A HEPN (higher eukaryote and prokaryote nucleotide binding) nuclease Las1 and a polynucleotide kinase Grc3 assemble into a tetramerase responsible for rRNA maturation. Las1 and Grc3 are highly conserved proteins and have recently been identified as core enzymes involved in processing and removing ITS2 spacer, which is a key step in the synthesis of 60S ribosomal subunit. Recent studies have demonstrated that Las1 is an endoribonuclease that contains a HEPN (higher eukaryote and prokaryote nucleotide binding) domain responsible for rRNA processing. Grc3 is a polynucleotide kinase responsible not only for Las1 nuclease activation, but also for nonspecific phosphorylation of the 5′-OH of the 26S pre-rRNA produced by Las1 cleavage, providing a signal for further processing by Rat1-Rai1 exonuclease.

Cleavage assay indicates that ScGrc3 can activate ScLas1 nuclease well for ITS2 cleavage, while CjGrc3 exhibits relatively weak activation ability for CjLas1 nuclease. To better understand the differences in the mechanisms of Grc3 activation of Las1 between different species, we also solved the cryo-EM and crystal structures of full-length CjLas1-Grc3 complex at 3.39 Å and 3.39 Å resolution, respectively. To be noted, the crystal structures were solved by molecular replacement method with the cryo-EM maps of Las1-Grc3 complexes. Structural superposition shows that the conformations of all Grc3 domains and Las1 HEPN domains are almost identical in the two complexes, while the conformations of Las1 CC domains are significantly different. Notably, compared with CjGrc3-bound CjLas1, ScGrc3-bound ScLas1 has a more compact catalytic pocket, which may explain why ScLas1 shows better ITS2 cleavage activity than CjLas1 in the presence of Grc3. In addition, His130 in the ScLas1-Grc3 complex active site and the analogous His130 in the CjLas1-Grc3 complex active site adopt two different conformations, which are similar to the conformations of His142 of CtGrc3-bound CtLas1 in two different active states. This observation may also provide a structural rationale for the activation of ScLas1 and CtLas1 by Grc3, as well as for the fairly weak activation of CjLas1 by CjGrc3.

>MHKSAFQALQGDIPTYEVNSSDEQDSDQDEEDVEQPSEPMHRLVSAPAASIHIEESKYISSNFSFDDDNTIYGHDYVIFGLKSNQNLIVKGQFVLEIQRGAIDINGVIYHSGVEPMKFINPSSSSIPLIQATQVLNSSLLENKESQENQHLFTPGYKSVIKLTNLDTHLESIGRVCPLFKNLFWQFDNFFAEDSLRLLDQYELAFSDYTFYPITKPDNTVSVIKHKNWMDVIKSLTELYSNDQSIKVIVIGGKNSGKSTFLRLLVQHMLSPTLQQLPINFMDLDPGQPEYSGTDCISLSKISEVQHGNHLSLTSTDSTQCHYVGFNSPKDQPTRYNLLVEQLVRSYESDGELKHESLLINTPGWIKGYGLELTRTLIERVKPTHVIYLNSGTLGVDIDIPKGTNLIPLQGSFNHSGSRYSSSQLRLLKTMAYFHKIDDFKFDFQPLLFSPPIQVSYGVSTGISALTHLKETGIGMDHLERSIEATIVGIFKVKRDHLEECELFNKGQLPLLPYKEFIKLSTEFFRLALVHSIDQEKKIMNLYIPQFRTLDLTKEAIIMVRGNTDLPIWEIASNEIVKRFKRQLPYITFEKGSSLEKKWKVRKNVQRRGQM[2x];>[2x]MNSHPRLTPWKSSDEVVYLKGLFFPADREQISRDELYRQYEEAISLVEMYSSRTRVSHILQSTAHLFSALMMLESFEGGLDDTVRLTASMTIIRFVNGLLDPNQQSQFAIPLHLLAKKIDLPSLFVEFRHSATHDALPSLEMCKTCVDRAIDWVWDHYWDGVLSIVEPQVETDDLEESLIKELKDLFKQYRRIRRQNITKLYKFGDSTPEGKEYWTCIAGIKDHADMANFYNVMIERIVSNKLKWEHLRALFEPMMNHFIHLKGWDFPLGLIDSMLSKNYEYSKFRGIDDTERAYLNDQEFKCAQKWIRWLAIEQIDRYDDVLVSKMIDTLGKTNHELNVELLEKLQSRFSADPVIKDKIQAKLTLIQRLSTDTKTKRMNNLEDIMSDLESLKKRAKVTPTLHIKSFESHPNWTPKPFGVI> MEYEWKPDEQGLQQILQLLKESQSPDTTIQRTVQQKLEQLNQYPDFNNYLIFVLTKLKSEDEPTRSLSGLILKNNVKAHFQNFPNGVTDFIKSEC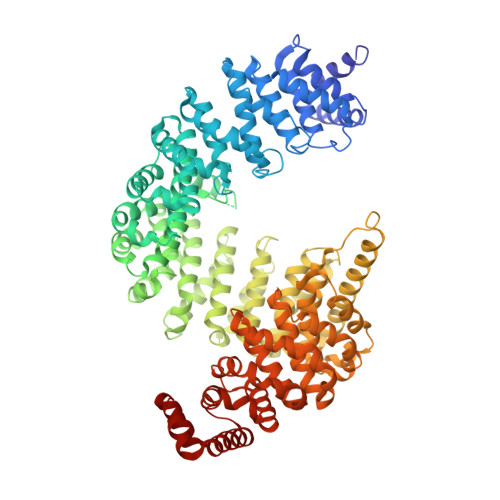LNNIGDSSPLIRATVGILITTIASKGELQNWPDLLPKLCSLLDSEDYNTCEGAFGALQKICEDSAEILDSDVLDRPLNIMIPKFLQFFKHSSPKIRSHAVACVNQFIISRTQALMLHIDSFIENLFALAGDEEPEVRKNVCRALVMLLEVRMDRLLPHMHNIVEYMLQRTQDQDENVALEACEFWLTLAEQPICKDVLVRHLPKLIPVLVNGMKYSDIDIILLKGDVEGGSGGSGDDTISDWNLRKCSAAALDVLANVYRDELLPHILPLLKELLFHHEWVVKESGILVLGAIAEGCMQGMIPYLPELIPHLIQCLSDKKALVRSITCWTLSRYAHWVVSQPPDTYLKPLMTELLKRILDSNKRVQEAACSAFATLEEEACTELVPYLAYILDTLVFAFSKYQHKNLLILYDAIGTLADSVGHHLNKPEYIQMLMPPLIQKWNMLKDEDKDLFPLLECLSSVATALQSGFLPYCEPVYQRCVNLVQKTLAQAMLNNAQPDQYEAPDKDFMIVALDLLSGLAEGLGGNIEQLVARSNILTLMYQCMQDKMPEVRQSSFALLGDLTKACFQHVKPCIADFMPILGTNLNPEFISVCNNATWAIGEISIQMGIEMQPYIPMVLHQLVEIINRPNTPKTLLENTAITIGRLGYVCPQEVAPMLQQFIRPWCTSLRNIRDNEEKDSAFRGICTMISVNPSGVIQDFIFFCDAVASWINPKDDLRDMFCKILHGFKNQVGDENWRRFSDQFPLPLKERLAAFYGV> MRGSHHHHHHGMASMSVSTASTEMSVRKIAAHMKSNPNAKVIFMVG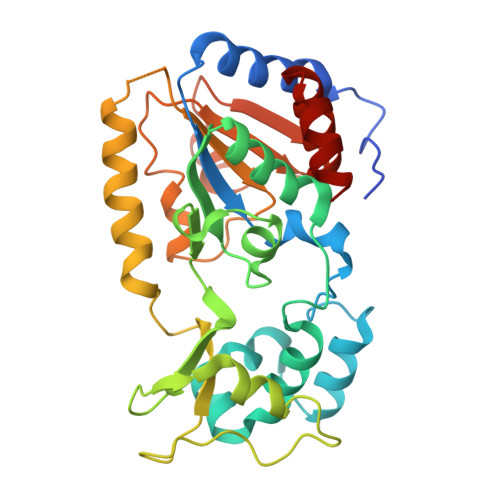AGISTSCGIPDFRSPGTGLYHNLARLKLPYPEAVFDVDFFQSDPLPFYTLAKELYPGNFRPSKFHYLLKLFQDKDVLKRVYTQNIDTLERQAGVKDDLIIEAHGSFAHCHCIGCGKVYPPQVFKSKLAEHPIKDFVKCDVCGELVKPAIVFFGEDLPDSFSETWLNDSEWLREKITTSGKHPQQPLVIVVGTSLAVYPFASLPEEIPRKVKRVLCNLETVGDFKANKRPTDLIVHQYSDEFAEQLVEELGWQEDFEKILTAQ3-[(2R)-oxiran-2-yl]propyl beta-D-xylopyranoside 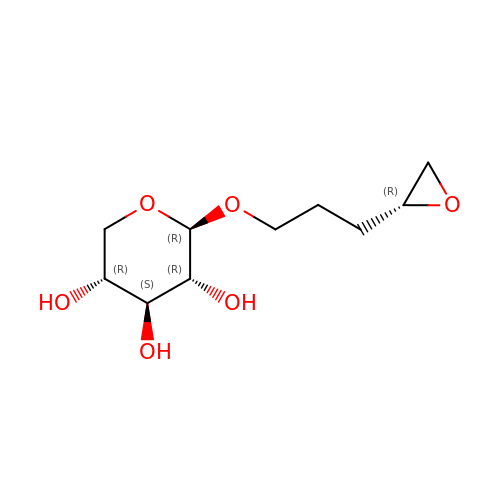| C10 H18 O6 | DMNHSULDBMDHLY-HOTMZDKISA-N Transmembrane Protease, Serine-2 (TMPRSS2) and TMPRSS11D are human proteases that enable SARS-CoV-2 and Influenza A/B virus infections, but their biochemical mechanisms for facilitating viral cell entry remain unclear. We show these proteases spontaneously and efficiently cleave their own zymogen activation motifs, activating their broader protease activity on cellular substrates. The protein domain organization of TMPRSS11D (and all other HAT/DESC subfamily members) consists of a small cytoplasmic domain at the N-terminus, a single-pass transmembrane domain, a Sea urchin, Enteropeptidase and Agrin (SEA) domain, and a C-terminal SP domain. The TMPRSS11D substrate-binding cleft consists of pockets of amino acids surrounding the Ser-His-Asp catalytic triad.

We reapplied this approach to TMPRSS11D by replacing its zymogen activation motif, LSEQR186 ↓ ILGG with DDDDK186 ↓ ILGG to create a dasTMPRSS11D construct, which greatly improved protein expression levels relative to the wild-type TMPRSS11D ectodomain protein which showed no detectable protein band (eTMPRSS11D). When the dasTMPRSS11D protein was overexpressed, purified, and concentrated to ~5 mg/mL, it underwent rapid autocleavage activation. The activated dasTMPRSS11D protein migrated on SDS-PAGE gels at a molecular weight of approximately 27 kDa and produced a single elution peak when purified further by size-exclusion chromatography. These data suggest that the dasTMPRSS11D protein underwent proteolytic cleavage to release its SEA domain, consistent with observations in HEK293 cells overexpressing full-length TMPRSS11D, where the serine protease domain was detected in conditioned media and the N-terminus containing its SEA domain remained attached to the cell surface. The dasTMPRSS11D crystallization trials were initially performed in the presence of high concentrations of nafamostat or 6-amidino-2-naphthol. Protein crystals formed in the presence of each ligand, but the final crystal structures contained no electron density matching the ligands. Instead, the zymogen activation motif of dasTMPRSS11D, DDDDK186-CO2-, was found occupying the substrate binding cleft of a nearby TMPRSS11D molecule within the crystal lattice. Interestingly, both the eTMPRSS11D S368A zymogen activation motif (yellow) and dasTMPRSS11D zymogen activation motif (magenta) adopted an α-helical structure oriented perpendicular to the face of the SP domain, whereas all other TTSP zymogen motifs were β-strand structures wrapped around the SP domain and/or the electronic density was poorly resolved around this region. The TMPRSS11D SEA domain was not resolved in either TMPRSS11D crystal structure. To facilitate the analysis of soluble forms of these TTSPs, we replaced their zymogen activation motifs with DDDDK; this delayed their zymogen activation and enabled protein overexpression, biochemical assays, and protein crystallization.

>[4x]AADQKSYFYRSSFQLLNVEYNSQLNSPATQEYRTLSGRIESLITKTFKESNLRNQFIRAHVAKLRQDGSGVRADVVMKFQFTRNNNGASMKSRIESVLRQMLNNSGNLEINPSTEITSLTDQAAANWLINECGAGPDLITDDDDK;>ILGGTEAEEGSWPWQVSLRLNNAHHCGGSLINNMWILTAAHCFRSNSNPRDWIATSGISTTFPKLRMRVRNILIHNNYKSATHENDIALVRLENSVTFTKDIHSVCLPAATQNIPPGSTAYVTGWGAQEYAGHTVPELRQGQVRIISNDVCNAPHSYNGAILSGMLCAGVPQGGVDACQGDSGGPLVQEDSRRLWFIVGIVSWGDQCGLPDKPGVYTRVTAYLDWIRQQTGIEFVEHHHHHHHH[4x]>MRGSHHHHHHGSMDKNIIIGAMTALITPFKNGKVDEQSYARLIKRQIENGIDAVVPVGTTGESATLTHEEHRTCIEIAVETCKGTKVKVLAGAGSNATHEAVGLAKFAKEHGADGILSVAPFYNKPTQQGLYEHYKAIAQSVDIPVLLYNVPGRTGCEISTDTIIKLFRDCENIYGVKEASGNIDKCVDLLAHEPRMMLISGEDAINYPILSNGGKGVISVTSNLLPDMISALTHFALDENYKEAKKINDELYNINKILFCESNPIPIKTAMYLAGLIE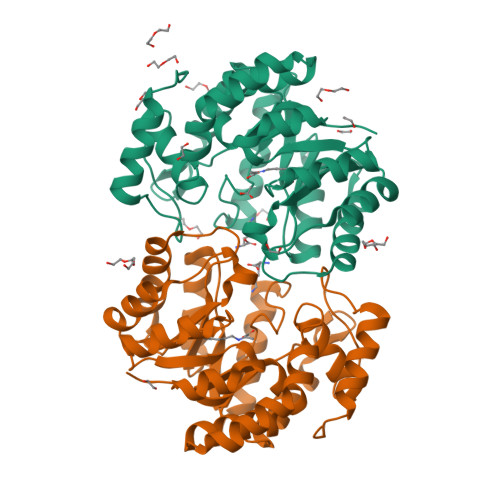SLEFRLPLCSPSKENFAKIEEVMKKYKIKGF[6x]>[2x]MDLQHWQAQFENWLKNHHQHQDAAHDVCHFRRVWATAQKLAADDDVDMLVILTACYFHDIV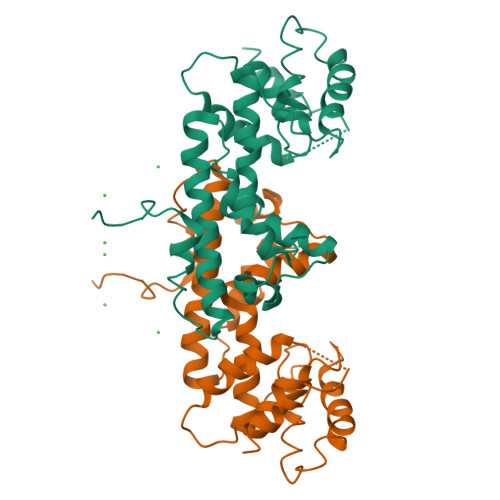SLAKNHPQRQRSSILAAEETRRLLREEFEQFPAEKIEAVCHAIAAHSFSAQIAPLTTEAKIVQDADRLEALGAIGLARVFAVSGALGVALFDGEDPFAQHRPLDDKRYALDHFQTKLLKLPQTMQTARGKQLAQHNAHFLVEFMAKLSAELAGENEGVDHKVIDAFSSAGLEHHHHHH> MSTTSMTAPATSPSRLESMRAASSTTSSKPAPTGPSKKSDAPAKTKRQDKPNVNSANDSNAADTGTAAAATRPDHGRRSRRTEDANWLNAEKPGNAYRPADKELSQNVKVVQDDILNREQAQREQAERAQRQKEKLEQHISESPAGFQAALPRLNELDVANSWDKLLRMMRSEYDMSCLTSCLARELDEDVAWNPEMLLVQLTSDMLDAAELQKDSGEAYVPVDASDIGQMTGGEVARKRKAKRTKAAGGAEGEPEKDTEMPATASPPPTSQAATSKTPRKKATTDPAAAEPKKTQTGKAQNAGPTSAGNSSLPQKGSAAGSTSGAAGGGGGSKTSAAPSTAKRDASKDANATKSSSSKKKTSKQVSK;> MFVYLSKRIAMPNGVKVTSIAWNDGQGWLACGGEKGLLKVLKVDGGPQGQRSGGLSSSQTLEGHDTTVDLVTWNQQYCKLTSSDVSGRIIVWVLHKGMWFEEMVNNRNSSRVVDFAWNPSGTKICITYEDGAVIVGGVDGNRYWGRELPYKLAKVCWGADGNSILFGTATGEVYVHDASSGEHLSQVEIKCNDGKAPSPLAGLSWHPAWVERPEPLATLAVCYQSGKLQLMTSIGDETPCNVDRDLPAHFISWNPSGTVLAVTAATPATEENGPGIVTQFFSTEGVHLRTLRVSGKQCGGITWEGGGLRVAIGVDSSVYFANVRPNYKYCYFKKTAVFAFTVPDKVEESVMFWNVNTNERRTKSVRGLQYMNACKDACVLISRPDTTQQQRMIQLVNAIGSPLETRFIDMELYTYDMNSSAVVCCGDESIYIWQFRDPSTAVDALDPISMQASRAESQERVIHVCDLVRGDTAPTMKVRSALTNDLISAMCVSETHMFVSLESGTLHVYQLSPLQLVSKYILFARAQSMSVNCNSTQLAVIHLGGITNVYCIEREKFSLVPCKADTIDGVELKDVWNLRWAVDDPHRFAVMEKTRMLVYNHGVAEEPVQSCANLCKFKSLKIRTLQLDELLLDPERPRKDYIVDFEAQLLRDMRAVLRDGTAKEAYEFAESHNTKKLWELLAEHTLFQLDFTYAEVAFIHCKDYAAIQFVKRVRSLDDPKKQLAEVNAYYRRFDEAERLYKDVDRKDLALDLRYRLGDWFGVVRLVQEGGGDEALLFQAWENIGDHYASRQKWSKAAQYYTQCRHYRKLARIFYIIEDYEMLTQLISMGEHDKELMVTLGNMLLTVGLAEEAAKAFIAANEPRMAVNGCVQVNMWNRAIALAKEHRLEDVGQLLEKYAKYLIHRERLTEAIELYRKAGKHDEAATLLAQLGKRAALRDALKAKKFYVLSALEVQKYRTTAIALNRDGVAVVSEMLNKDRSTVSERTLDAAWRGAEAYHFLLMCQQQMADRNFKAALVLAMRLIEYDDLVAPVDGYSLIALTAYLVKNFGLCSKAFARLEQAERNDEAGGVAAAATTQLENFSLDLDVTHRTMASTCGGSTGGSTGMLSGGGGSALSGTTTSLQLTNPGKGVTRMAPMTYPTVSLRDPPRPFADLARHIFMTHSPVDTSVDSVPCPTCGSFNKEWAQRCIKCQQPFNTCIVSGCAIVSEDGAWQCSVCHRKALEAVVDKYRNCPLCHTPRKGRMRRGI;> MHTSVRWSETADAVKGIRPPVNSLCYSPSGDYVVASCGVRVLVYAASTGTLLHSLMGHQDTIYCVDYSSDGKNFASGGADRTVIVWSSQGEGIVKYQHTEAIQALAHNPTSSQLASVSSVDWGIWSPEQPKVSKYSLPSKGLCAAWTPNGKTLAIGMLDGTVMMLSKTSEEKVIIRRPAPVWALAFTPLRENGIDVLAIGSWDQRLSFYNLSGTAVGRERELDFDPCSVSYFNDGEYILLSGSDHKVTLFTKDGNRLIELASADDWIWSARQRPRQKQFCYGTNDGTISCIDITISTVHTIYDDQYVFRKDMTNLVVHQLLVDRKMVIPCNEYVQKIATFLDKLAVQLQERVIVFEFFYDDDRTMRYQDIAQIRRRLECSLLCVTTGAIIVSNDKRITMYDFQGNKRREWSMESPVQLMKVVGGMEGREILLVGLNGGQVMKVFVDNPFPTLLHKGTAPVKSAELSSSRSRLAVIDSTNTLQVLELGEKNELLFSEDNVTAVAFNIDVDDNIAFTTGDNTLHIKTGSLPAYQQAVRGIVVGFKANHVFNLHYSNMMVLDVPHAHALYKYVEMRDFDRAYEVACLGVADADWKMLGLHAMSQLRLDIARKAFTHIQDTKLVELLKSLELRRRQSGAEDGLSLTLGKASGTPDTVEGPENKGYGSTNGELAAARVAAKDSVLYGSILAFQGKYNDAARQFMKTGCELKAVEMYCDLKMWDNAKKICTDEKVLKDLIRQQARWAEESQNFVEAASLYESCGDYAKAIGMMGQAGQVEKLMKMCRSLPTSEVTLITECANFFRKHNAIPFAIEAYEKVQDHQALIGIYVAKGDWRNAFTILEKTPTLAREVYVPWATWLADNDKFDEALEAFRAAKWPKEAMRLMETLATNSVTCRKFRDAAFYYIHLAEEYGRFEETEKPTDVEKAARIRRSKECVRRADIYYAFSGVYAHTTQPLPYNELSLFRTAKYLFGMCAESAIPINVGKGAILYTLSRIANRLEMVRTARAVFEKLQGVILPVSMMEQVDIETLLVRSKPVKDRDELLDRCFRCNQLIAQLPMAGDRCPNCFHPCVRSFVNFECLPLVEFVLADELTDEEAERIIVSGVGRRRSADDENSKDHSDGADAKAKEWKSDNGANVISFDDGNIDYEIDQQLVAMGRSKAAANKGNDPFFTQLQYVLRPGRPTATYQPFVASADILKGFRRDEVFIVRPRYGTLPVPNRYYRLMRSDVSVCLCNGCQHFFIAEDYEAECMRGSGCPLCRYRPGKQVSRSMKQILFDMETAAAASKTSSAAAAL;> MQPSSSFLPDVWMAVTREPHIPEITPLSRILAAAAISTYSRQVEYDLDTGCKKKRTAPPPSPPPPSSPPPSPRLTLANAAAMTTTILRTNYALLLFYVREKYWHHAEEVCLSVIQSTDDHMFRVWRALTLERQGMANDAIREYKAVESRRTTAVPALMGMQLIYKHNRDQEGVAQTEAKLDGFEIAANMGGWVQAAALCWAMGDINAARDILLRFTDNEAAMAYRDEYTNYGTIRGWVDLLSGRGALLEKAGALFTSVMDMEEAQYSYFQADNESGSGSRGTTKWIDLNAALGYVAFLERKTQLAKAQSLLDRLFVLYPNCSIPPLVGKARLLMQAEDWEQAIEVTHRILAHDKSNVEALALEALYAMAKDTRHDAAPVRVRRLLDAVRAKEPRNVALLHQFALVFSRLAGDRLDLLSLTTQFSDMAYALDSRNGDVLCGLGYQQLYRHDDKAATETFRKAATLTDSLDPLLGTVTCLLRQGDMEAAATQLQLCNQLQPAAQRNAELSMLNAQLRWHRRGMEEETAVLRYLDQAAEAIKQDVKERAGVGMEVYVHLNAPVALAIAHAYIMHCRNEPPDPMFKHADVVGEKCGRHLEFIVQHLPACMEAQLMLAKVWFVTGEVRKAQNLLKSTLIVQEQPLPDAFLLSSQICQYMGDTKLACQALAQARTLDFSLQEKPLYNLLLGTVKGTTGEYAEALASLQRAYNTVKSAATAPSAGKPTNPLSVPETVTLYLQLAQAQLRVRDVDAARETLTEAALKFRGSAQIGRVIIAQAMLAARTDVDKSIELLRQVSSKSEFYIAAHSQLGKLFLTHKHNVAMYIQCFQEMAESVPSAQSYVELGEAYTTIQEPEQAIAAYEKAKALSPSSSELSVRVGRALVAAHDYAKAIRYYQDALVTDPHLSIVRADLATLQWRLGHIEEARETIVASPVYELPSTDGAGAGVASAAAAGSAEAVGTAIERINLYLLLYKVLRDQPWTVPLSEEGTAAADSDDNHGDAALTALLTARSLQRRLLEHQLRTTEAPEVITEQRVVMSRICTEAGARCIYSTPAPPPFSVVMTDKKVEAAAALAVQSAIASRLTNAREYLREAIAFDESNERAQLESAQLCYRTGDTEGCEQHCTTVLRMAEGSANTADAAILLANLYTEQNRDEDARNMFEDLLRKTPQHYEALVYYLILLYHAGQLPEAKEALERAAAAVPIGQRADPGLSYVRGLYEHLCNNNAEALRHFNLARLPAGNPWCTRALVRMIRIYLVPTTQDLWVRGTSPAAAAATAVADPPRAKEQQQKSATPGKVPLAAATTGSTELHDNIRHAEQLLLLLPVHSEERRILQAYCTMATRRPEELETALHLFLECIVAAETGGVSAAMTAEKNGGSGSPKKTAAEERKQPRRGKGGDSDDDEDLQLLASMHEAAAELAQRSSGNSTATLAFALQCKVIHPEAFLGLAICLFISGQETAARNVLARLLESKDITTKMSAMKQAEDKEDAASKDAASKEAAEPAAPMVLSPPIAILTCSEDDTIERAMLFEAYMDTQEGRLKDARFVLQQVLSANEGCSSAWNELGLIYERNQKHKNASQCYQKAWKLVQEADPDVGYKLGFNYLRGGQPVKAIDVCKRVLTHHATYPRIEADIMDAAYSMLRP;> MSLFVVNAPGHEGQLKEQLIVAHKRRPLLATAWVNPPSVLITNSEGEVLTQVADPPGSTGRTHQPTALTWHPNEELLVIGWSNGEMSLWSMPSVSSLALGEDYTTAAARSAVQLIAAKAATQSSAEGATREHASGAVVASEWSTRGLYLVSASQQRHVVMWMLEKIPAETSVTFKLKPLWSVQSREPVARIIHVPSKASHPSTAFKLNNGATAAAAAEGGDDDISFLLADGGTSVTAINEDQQLFPCVTQQEQIASVLYDAATRTLVTLTTTSMIEVYAVGEDIKGTSTLRRKLSAPATTPTVSTTTGERIAMSMVWASPGVVAFGSGDDRLRILDLSSGSLDVLLLPQPDLHVSSLATFAAKGTMIVGTVEGFLVVFQHHAASLLTSRHVSVARETVTSSSPFAPAATEASQWEAMTVHQVGKCVDRVVLTALGDVALCCGGSELQVLHEIIRKRAWDGVAAATQISSDMVVIESITGCQCLLQNKGNVHGVSIAFPNIALWNGSQIDFYMIDEATSEITFINFVLTTSPAFAIHREGLIYVKGNRIVFETMQLAPIAQMTFTESEGVPVIMDIMNDYLVVVSSKNYLRLARISTRDLQQLGPARPLTFPSILQPDAVEASSGASEMTPFVEDISTLEVSVSGARVNAQGRRVALMSTLGPLALPDTRIWVYDSDTDKMSFFDFGSRNEIPNSVYWNTPEPNTTTVGEFEYILLACETYQIHMDDKKSASEEAESPKACTDTTNDGNKIADHPVGQENLPEALPDMENYAEKKAELEDARRESVGTTNYVSQRPHNIVTFFATHDGLVLQNFAPLRRYQICLVGLTIPDFLLASVKINGDPNNAEDYVIEQKRLRDFEGLKSDKDVAVREALMKFSYYATIGNMDEAYRCVKSIKNPAAWQGLARLCVTSGRLDVAAVCLATMEDCVAARALREAKEDYPDDQDVQLATLALGLSMTEEAVELLRKSKRYDLLTDVYMACGKFEHAQRHSERFDRARIRPVAYKYAQFMESLQNMDAAIMWYYNAKCASTDVPRIFFQTNRMHELRQLMMIQSQPPSPTAGDSAQRPQPGIGEQQSTFATIFPQNRELLLWWAQHSERRHNVQEALRFYNAGEDVYNIVRILCSLTPPKLDSALQLVNKEMDKAKMRFQQQQAFAATASARFGDDDHGEPDPVGSAYFVAQLYERQGDDQLALQYYQAAGAYRSGVRVAWKMEQYGVVANLAMKSSDERLMLETAMALEKHQAYDKAVQLYRRIGAVQCALDACVQGGLYETLHEVSAAFASGSTDPAVFLGMADHFQSESDYQKAVEMLLFAKHFEEALKLCETQNATLTEEMAESMTSNIGELSMEERQAVLRRVAHIAKDQGRWSLACKKYTQAGDRVKAMRMLMRGGETEKVIFFANHSRNVEIYTMAANFLQSQNWSADANIYKSIVLFYTKAKAWMNLLAFYESCAQLHIDENRNYPEALRALEDCIAMAESVRGGKANIEMEKVEQLKQRVEILKAFVKAQKTVDSMVVAERGSVAEKAKADSVIACCSGLIKRSRPSSPDHSLIQDALRIGDVFALMVRFYFDKLGEPHNALKVMESMPKHGADPQLFIEADYMERVCQANGKSLANVLPGGIATEAPGAVWEGARKFSTDTRRSSVIDEVDRVV;> MVLTQQFVISNADLGRGHVVEALHPSSPLIALAGSKGRVLILNKTGKVEHQLPMQNVVAMEWECSTDTLAIITSSSSDVHLYTHRTRQTDTIDTKLKDLCFVCWSQSQPLFAIGSKSGQFVLYNRRTLRLVPVADTHKQRLISGMWVPAQDSRLLIISEDPSLSISDAEGKVLTTIPLPSVPKSVCVSGMANSPKSSSFAAVNLDNTLLIVDLRSYATAAGQFNSALGQITCLTAGINGEFLAGFASGTVALLDLAGSEVRLRGSLRLLKNAVEMVNFGEGSGVVAAVADNRVGLLRITEDGIAPTGDEASLESERGVPDLLAWSRDGQQLFVGTNQGNVTVFTLKVLNVSASYGTLVFSFTSNRTIGVKNLQDNRVVCTVPVNSDPAFISAGMAMLAAGVNNQVSYYEYFIPNSLPYPMVDPAKNVSQSSQQAHSVFLRTVEYPSPVTDLKVNSNLAAVVYDGRVQLSPIRDTPEAAAPVYFPESGDTRLVSIALSEVFFLYATTSRVSVYALHNLQQVATFTCNTGLKRAFANPACTRVAYVDDSSELFNVNLVTEVANKAEGYDPDQKMVLWDQAEATVFITYDSEKC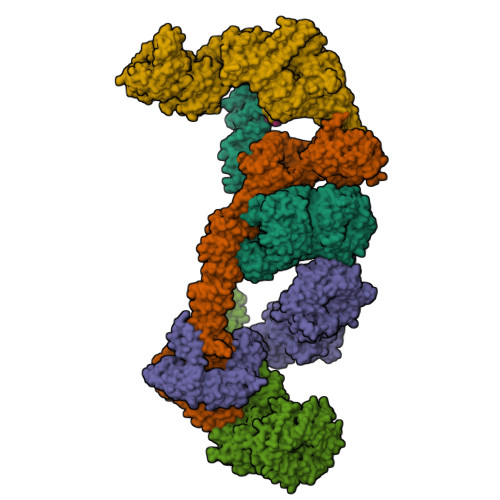ATFVNTPHSRHGATCESVLVKDSSEDNLYTPLPPGYTPVTLFRGTVVCQTPNGTLETVPLQTHNNIFLRTPNAEAFYNNFSLNRLRWSSNNITSPQEAEDLAVKSLHMLDVELAIRVYRQLSQPSLVLCLEKIRHIHEKNLLLGHVSMIMGYMKDAQNFFLRSSQPLRALEMRRDMMQWERALTLAEQLAPEEVPIISRDYAQHLEYRGVYAKALEMYQKGLRQLPTGHASTELSVTVQEVERHNEQCRQGAARSQIRIGNIADAMKTVKESSEVSFVKECAKLCEENQKHEEAAQLYEKAGDIERAATIYIERCKNLKAAERLLPFIKSRNIIGIYARGKEAEGAFVEAEKAFAQAEDWDNAVRLRIEKLNDLHGAYVIVRQTRSANAAALVAKKCTAQKEYGTAVEFLVLAKSLDEAFELAKTHDCMFNFESALLNQVQLKDGIAPLSNQADFTMIAEYYDNDGKAGQAGMYYHISGHYAKALNKYLESGQPEDIEKAVEVVGKAHSDSLTNKFIDYLMGETDGEPKDPSYIFKLYLAMGSYEKAAKTSVIISAKEQEIGNYKSAHKTLVEAYRILQQRNMHVSNDLRRALMLLHSYIIVKDLLKIMKDDDTACRMLLRVSRNIQKFPKHITTIVTTTVLQCLKSNFKKSAFEYACYLIQNEKHRAEMTEKSRKKIEGIVRRHSKDDAVDPVEPMLPCPYCDAPVAETELDCGACKNTIPFCIVTGKHIVKSDYTSTPCCGFPAIYSALMTRLSGTLTCPMCEATIDISNVNRETNPELKALL Trichodysplasia spinulosa-associated Polyomavirus (TSPyV) was isolated from a patient suffering from trichodysplasia spinulosa, a skin disease that can appear in severely immunocompromised patients. TSPyV has a 5232-nucleotide dsDNA genome encapsulated in its non-enveloped icosahedral capsid made up of the proteins VP1, VP2 and VP3. As is typical for polyomaviruses, the TSPyV VP1 monomer adopts the iconic jelly-roll fold with a conserved core comprising two β-sheets that are formed by strands B, I, D, G and C, H, E, F, respectively. We demonstrate here that the skin-tropic TSPyV binds sialylated glycans in a binding site formed by the BC2-loop on top of the VP1 protein that is not utilized by any other structurally characterized member of the polyomavirus family.

Following cell attachment studies, we determined high-resolution X-ray structures of TSPyV VP1 pentamers alone and in complex with glycans bearing α2,3- or α2,6-linked terminal Neu5Ac. For these experiments, TSPyV VP1 was recombinantly expressed in E. coli. The VP1 protein forms the characteristic homopentamer but cannot assemble further into viral capsids due to N- and C-terminal truncations of the expression construct. Extensive loops connect the strands on the top of the VP1 pentamer and are named BC-, DE-, HI- and EF-loops according to the strands they connect. The long BC-loop folds into two different directions on top of the protein and is divided for clarity into BC1-loop, BC-linker and BC2-loop. The comparison of all seven structures reveals that TSPyV VP1 does not differ drastically in its amino acid sequence, length and fold of the surface loops. The TSPyV VP1 structure superposes on the BKPyV and JCPyV VP1 structures with small root-mean-square deviation (RMSD) values of about 0.8 Å (calculated for Cα atoms of the VP1 monomers). The groove forming the binding site for the terminal sialic acid in VP1 of BKPyV and other polyomaviruses next to the HI-loop is still present on TSPyV VP1. With Y68 and L276, the equivalent region of TSPyV VP1 is similarly hydrophobic. However, while the carboxylate group of Neu5Ac is recognized by two hydrogen bonds from side chains of residues S274 and T276 in BKPyV VP1, similar interactions are not possible in TSPyV as the recognition of the sialic acid carboxylate group appears to be electrostatically hindered through residues D280 and D282.

>[10x]GSHMASKGNIEVLNLVTGPDSITTIELYLNTRMGQNDESKDNYGYSEKVTVANSSDQDKPTSGEIPTYSTARINLPMLNEDLTCNTLTMWEAVSVKTEVVGVSSLVNVHMATKRMYDDKGIGFPVEGMNFHMFAVGGEPLELQFLTGNYRTDYSANDKLVVPPIKHQSTQGLNPHYKQKLTKDGAFPVECWCPDPSKNENTRYYGSYTGGQSTPPVLQFTNTVTTVLLDENGVGPLCKGDGLYVSCCDIVGFLVGKDGDMQYRGLPRYFNILLRKRTVRN The COP1 E3 ubiquitin ligase is a central signaling hub that integrates inputs from plant light‐sensing photoreceptors. COP1 contains an N‐terminal zinc finger, a central coiled‐coil, and a C‐terminal WD40 domain, which is essential for proper COP1 function (Deng et al, 1992; McNellis et al, 1994). COP1 regulates gene expression and plays a central role as a repressor of photomorphogenesis by directly modulating the stability of transcription factors that control the expression of light‐regulated genes.

We mapped putative VP motifs in all these proteins and assessed their binding affinities to the COP1 WD40 domain. We could detect binding for most of the peptide motifs in ITC assays, with dissociation constants in the mid‐micromolar range (Figs 4A and EV4). Next, we obtained crystal structures for the different peptides bound to COP1 (1.3–2.0 Å resolution, see Tables EV1 and EV2, and EV4) to compare their peptide binding modes. We found that all peptides bind in a similar configuration with the VP forming the center of the binding site (r.m.s.d. between the different peptides range from ~ 0.3 to 1.5 Å, comparing 5 or 6 corresponding Cα atoms). Chemically diverse amino acids (Tyr/Arg/Gln) map to the −3 and −2 position and often deeply insert into the COP1 binding cleft, acting as anchor residues. C Superposition of the VP peptide binding modes of the HY5 (green), COL3 (orange), and STO (gray) peptides depicted in ball‐and‐stick representation when bound to the COP1 WD40 domain as observed in their respective X‐ray crystal structures. As for UVR8, COP1Lys422Ala showed increased binding affinity for some peptides such as those representing the COL3287–294 and CO366–373 VP motifs, while it reduced binding to others, such as to CRY1544–552 and CRY2527–535. These observations may be rationalized by an enlarged VP‐binding pocket in the COP1Lys422Ala mutant, increasing accessibility for the COL3Phe288 anchor residue, and potentially abolishing interactions with CRY1Asp545.

> GAMTFTRYSRLRVIAEIRHGDIFHSANIVSSIEFDRDDELFATAGVSRCIKVFDFSSVVNEPADMQCPIVEMSTRSKLSCLSWNKHEKNHIASSDYEGIVTVWDVTTRQSLMEYEEHEKRAWSVDFSRTEPSMLVSGSDDCKVKVWCTRQEASVINIDMKANICCVKYNPGSSNYIAVGSADHHIHYYDLRNISQPLHVFSGHKKAVSYVKFLSNNELASASTDSTLRLWDVKDNLPVRTFRGHTNEKNFVGLTVNSEYLACGSETNEVYVYHKEITRPVTSHRFGSPDMDDAEEEAGSYFISAVCWKSDSPTMLTANSQGTIKVLVLAA;> XGFGVVPSFY>MKLYYTPGSCSLSPHIVLRETGLDFSIERIDLRTKKTESGKDFLAINPKGQVPVLQLDNGDILTEGVAIVQYLADLKPDRNLIAPPKALERYHQIEWLNFLASEVHKGYSPLFSSDTPESYLPVVKNKLKSKFVYINDVLSKQKCVCGDHFTVADAYLFTLSQW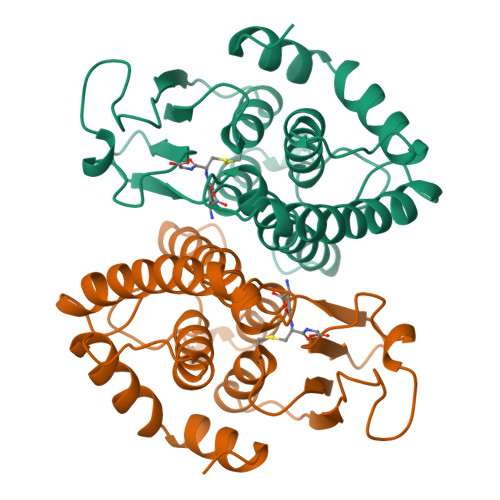APHVALDLTDLSHLQDYLARIAQRPNVHSALVTEGLIKE[4x]>MSIIAINENGFLDKIKGRNPLFTCVISSIETTLSIPISGVHRDVIKYTPSADVELVFYGKSLTLKTPPIDATGSPTPATITRACVELKNIKNLHIDAGAFVKPKIPFIEIDEKPTGRIEEGKAMNNSKELYMKGYLLGKNLDAELLIVGESVPGGTTTALGVLLGLGYDAEGKVSSGSINNPHELKIKVVREGLKKAGINEKSSVFDVLNAVGDKMMPVVAGLAISFAERNKPVILAGGTQMSAVLAVIKEINKKVLDKNLIA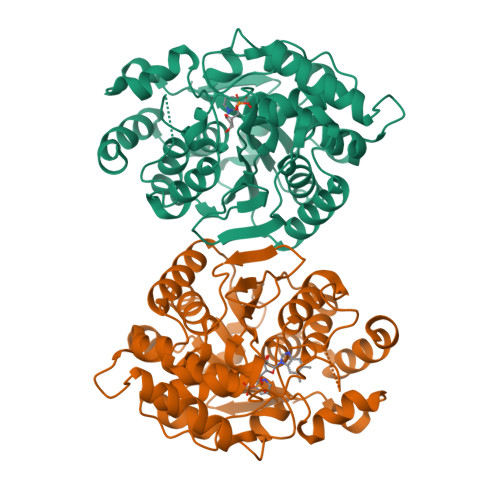IGTTEFVLNDKKGDLKGIVEQIGNVPVLASKFYFEKAKIEGLKNYCKGSVKEGVGAGGIAVYSIVNDLEPTKIREFIENKFYEWYKE[2x]~{N}-[(1~{S})-2-azanyl-1-[4-(hydroxymethyl)-1,3-thiazol-2-yl]ethyl]-5-[3-fluoranyl-4-(trifluoromethyl)phenyl]-1~{H}-pyrrole-2-carboxamide 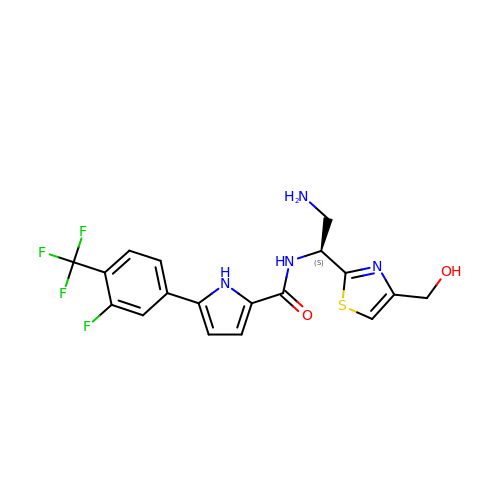| C18 H16 F4 N4 O2 S | ZKOITYDZLQYLNI-HNNXBMFYSA-N Phosphoserine aminotransferase (PSAT) is a pyridoxal 5′-phosphate-dependent enzyme involved in the second step of the phosphorylated pathway of serine biosynthesis. PSAT catalyzes the transamination of 3-phosphohydroxypyruvate to 3-phosphoserine using L-glutamate as the amino donor. The pyridoxal-5′-phosphate (PLP)-dependent transamination reaction catalyzed by PSAT, which necessitates a lysine residue in the active site, has two reversible half-reactions. In yeast S. cerevisiae, the SER1 gene encodes PSAT and yeast cells supported by fermentable carbon sources, mainly by the glycolytic pathway, to synthesize serine and glycine.

Therefore, to elucidate the structural features of fungal PSAT, we determined the crystal structure of Saccharomyces cerevisiae PSAT (ScPSAT) at a resolution of 2.8 Å. ScPSAT exists as a dimer in the asymmetric unit and appears butterfly-shaped. Fifty-three N-terminal and seven internal residues (i.e., Lys 218, Asn 219, Ile 220, Ser 268, Ala 269, Tyr 270, and Asn 271) could not be modeled due to weak electron density. The ScPSAT monomer consisted of two domains: a large domain (residues 54–293) and a small domain (residues 294–395). Furthermore, the large domain exhibited a Rossmann fold that contained central seven-stranded β-sheets (β1–7 with strand topology 3-2-4-5-6-7-1) surrounded by twelve α-helices at the periphery of the domain. The small domain folded into antiparallel β-strands, β8 and β9, flanked by four α-helices, α12, α13, α14, and α15. Moreover, the halide-binding site and gate-keeping loop were located between the large and small domains. For instance, helix α9 existed only in ScPSAT, whereas human, plant, and bacterial structures exhibited an unstructured loop. The HsPSAT structure contains a cofactor PLP, whereas the ScPSAT structure is an apo-form. Due to the lack of PLP bound in ScPSAT, the N-terminal region might be not stabilized in the structure.

>[2x]MSLEREEPQHFGAGPAQMPTPVLQQAAKDLINFNDIGLGIGEISHRSKDATKVIEDSKKHLIELLNIPDTHEVFYLQGGGTTGFSSVATNLAAAYVGKHGKIAPAGYLVTGSWSQKSFEEAKRLHVPAEVIFNAKDYNNGKFGKIPDESLWEDKIKGKAFSYVYLCENETVHGVEWPELPKCLVNDPNIEIVADLSSDILSRKIDVSQYGVIMAGAQKNIGLAGLTLYIIKKSILKNISGASDETLHELGVPITPIAFDYPTVVKNNSAYNTIPIFTLHVMDLVFQHILKKGGVEAQQAENEEKAKILYEALDANSDFYNVPVDPKCRSKMNVVFTLKKDGLDDQFLKEAAARHLTGLKGHRSVGGFRASIYNALSVKAVQNLVDFIKEFAEKNA>[3x]SMRSSSHSSRRAKSVEDDAEGHLIYHVGDWLQERYEIVSTLGEGTFGRVVQCVDHRRGGARVALKIIKNVEKYKEAARLEINVLEKINEKDPDNKNLCVQMFDWFDYHGHMCISFELLGLSTFDFLKDNNYLPYPIHQVRHMAFQLCQAVKFLHDNKLTHTDLKPENILFVNSDYELTYNLEKKRDERSVKSTAVRVVDFGSATFDHEHHSTIVSTRHYRAPEVILEL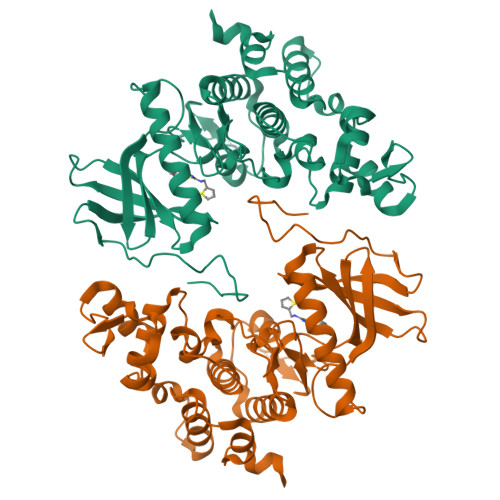GWSQPCDVWSIGCIIFEYYVGFTLFQTHDNREHLAMMERILGPIPSRMIRKTRKQKYFYRGRLDWDENTSAGRYVRENCKPLRRYLTSEAEEHHQLFDLIESMLEYEPAKRLTLGEALQHPFFARLRAEPPNKLWDSSRD>[8x]MRKIVVAAIAVSLTTVSITASASADPSKDSKAQVSAAEAGITGTWYNQLGSTFIVTAGADGALTGTYES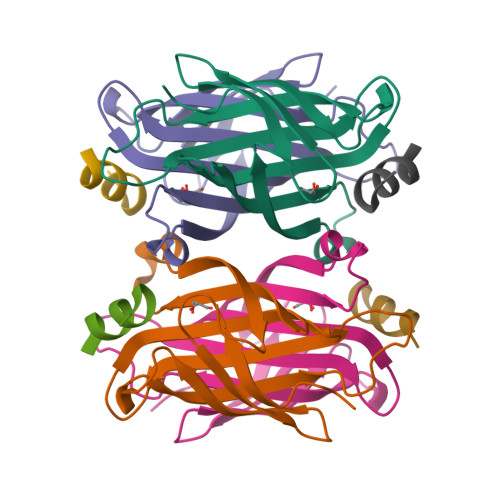AVGNAESRYVLTGRYDSAPATDGSGTALGWTVAWKNNYRNAHSATTWSGQYVGGAEARINTQWLLTSGTTEANAWKSTLVGHDTFTKVKPSAASIDAAKKAGVNNGNPLDAVQQ;>[8x]GNSFDDWLASKGX>MASNQQDVVKELNQQVANWTVAYTKLHNFHWYVKGPNFFSLHVKFEELYNEASQYVDELAERILAVGGNPVGTLTECLEQSIVKEAAKGYSAEQMVEELSQDFTNISKQLENAIEIAGNAGDDVSEDMFIGMQTSVDKHNWMFK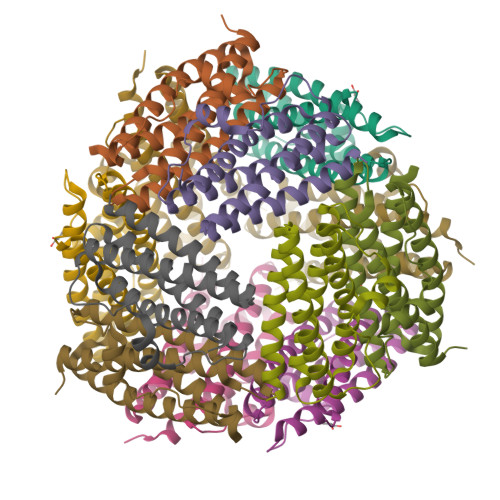SYLSLEHHHHHH[4x]> SSTHRKFGGSGGSPFSGSGLSSIAVRSGSYLDAIIIDGVHHGGSGGNLSPTFTFGSGEYISNMTIRSGDYIDNISFETNMGRRFGPYGGSGGSANTLSNVKV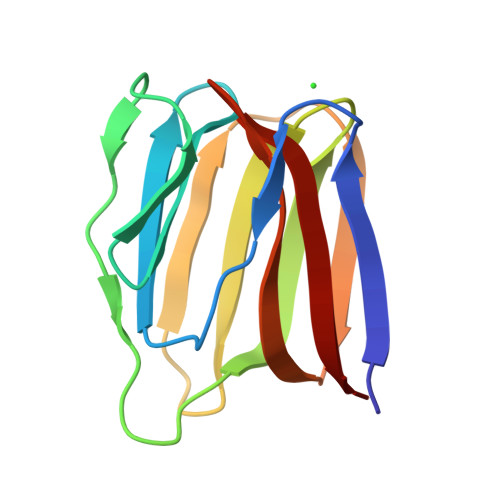IQINGSAGDYLDSLDIYYDN>MLDNSFYTAEVQGPYETASIGRLELEEGGVIEDCWLAYATAGTLNEDKSNAILIPTWYSGTHQTWFQQYIGTDHALDPSKYFIISINQIGNGLSVSPANTADDSISMSKFPNVRIGDDVVAQDRLLRQEFGITELFAVVGGSMGAQQTYEWIVRFPDQVHRAAPIAGTAKNTPHDFIFTQTLNETVEADPGFNGGEYSSHEEVADGLRRQSHLWAAMGFSTEFWKQEAWRRLGLESKESVLADFLDPLFMSMDPNTLLNNAWKWQHGDVSRHTGGDLAAALGRVKAKTFVMPISEDMFFPVRDCAAEQALIPGSEL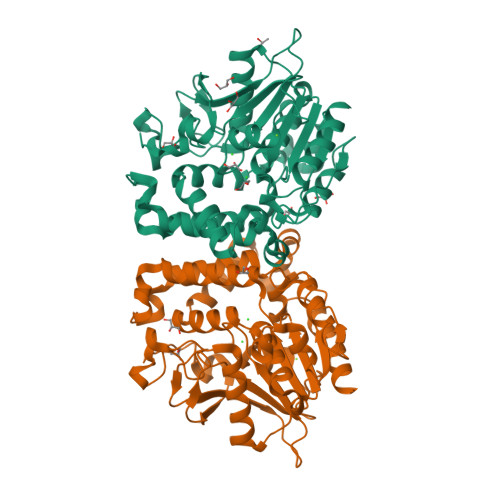RVIEDIAGHLGLFNVSENYIPQIDKNLKELFES[4x]>SKVVYVSHDGTRRELDVADGVSLMQAAVSNGIYDIVGDCGGSASCATCHVYVNEAFTDKVPAANEREIGMLE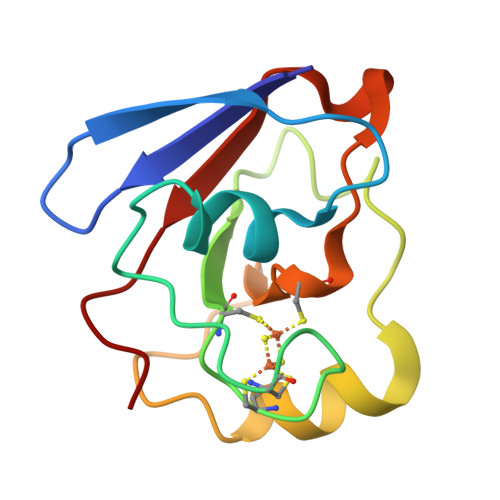SVTAELKPNSRLCCQIIMTPELDGIVVDVPDRQW[3x]> ETGESPPVFIKKPVDQIGVSGGVASFVCQATGDPKPRVTWNKKGKKVNSQRFETIEFDESAGAVLRIQPLRTPRDENIYECVAQNPHGEVTVHAKLTVLREDQLPPGFPNIDMGPQLKVVERTRTATMLCAASGNPDPEITWFKDFLPVDPSTSNGRIKQLRSGGLQIESSEE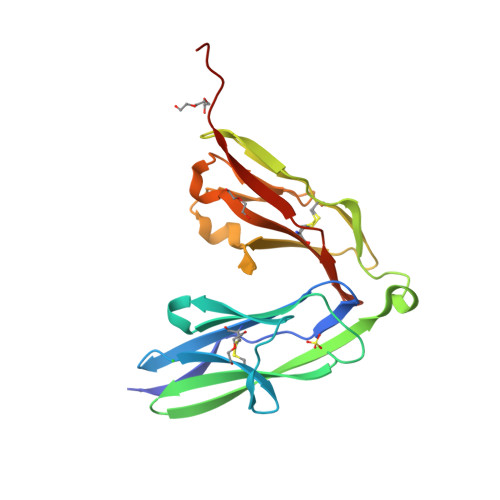TDQGKYECVASNSAGVRYSSPANLYVRVGTKHHHHHH>[2x]MGSSHHHHHHSSGNEIKLILQQYLEKFEAHYERVLQDDQYIEALETLMDDYSEFILNPIYEQQFNAWRDVEEKAQLIKSLQYITAQCVKQVQVIRARRLLDGQASTTGYFDNIEHCIDEEFGQCSITSNDKLLLVGSGAYPMTLIQVAKETGASVIGIDIDPQAVDLGRRIVNVLAPNEDITITDQKVSELKDIKDVTHIIFSST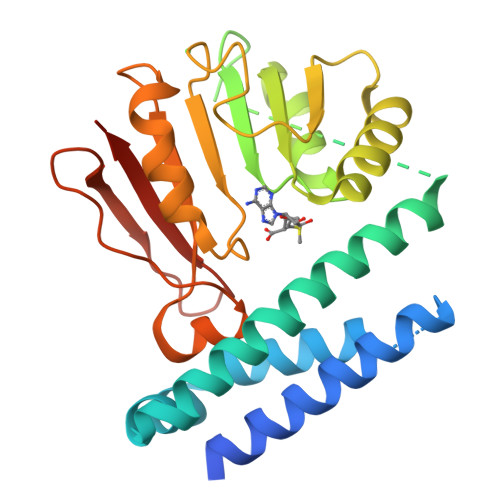IPLKYSILEELYDLTNENVVVAMRFGDGIKAIFNYPSQETAEDKWQCVNKHMRPQQIFDIALYKKAAIKVGITDV To investigate the architectural parameters that dictate the substrate specificity and site-selectivity of a Rieske oxygenase catalyzed reaction, we focused on two Rieske oxygenases, SxtT and GxtA, which are involved in the biosynthesis of paralytic shellfish toxins. These enzymes share 88% sequence identity with one another and selectively install a hydroxyl group on adjacent C12 and C11 positions of a tricyclic saxitoxin scaffold, respectively. Each structure showcases an α3 trimeric architecture, and each protomer of the trimer contains a Rieske cluster in the N-terminal domain and a non-heme iron center in the C-terminal domain. The trimeric quaternary architecture places these metallocenters within electron transfer distance of one another across the subunit-subunit interfaces.

To investigate how the native hydroxylated substrates bind to SxtT and GxtA and to identify global architectural differences between these proteins, we solved the structures of SxtT and GxtA with β-STOH bound, as well as that of GxtA with STX, bound to 1.79-, 1.79-, and 1.74-Å resolution, respectively. In SxtT, the presumed native substrate β-STOH shows slight deviations in its position in the active site relative to that observed with ddSTX, but it maintains interactions with Arg204, Cys228, Gln226, Ser230, Asp239, Tyr273, and Thr276. The differentiating feature between β-STOH and ddSTX, the C12 β-hydroxyl group, forms only one additional interaction in the SxtT active site with Tyr198. This interaction is mediated by a water molecule and Tyr198, like Cys228, Asp239, and Tyr273 is conserved in GxtA. The most significant structural difference between these substrate-bound structures of SxtT and GxtA is the orientation of a loop that connects the β13 and β14 strands of the C-terminal iron-binding domain. In SxtT, this loop extends toward the active site and interacts with β-STOH as well as with non-conserved residues Ser230 and Glu272. Two of the corresponding loop residues in SxtT (Val206 and Ile209) are hydrophobic and unlikely to reside on the protein surface or form similar interactions with the corresponding surface residues Pro233 and Glu234. Accordingly, whereas both orientations of the GxtA loops reveal an open path from the surface of the protein to the substrate-binding site, the SxtT loop, which is tucked into the protein interior, blocks the analogous path in the crystal structure. Outside of considering the overall loop architecture, in SxtT, the loop is important as it interacts with a bound substrate using residue Arg204. This Arg204 interaction, coupled with additional interactions that are formed between active site residues (Thr276, Gln226, Ser230, Asp239, and Tyr273) and the guanidinium groups of the five- and six-membered rings of β-STOH, ensures that three regions of ddSTX and β-STOH are recognized by SxtT.

>[3x]MTTADLILINNWHVVANVEDCKPGSITTARLLGVKLVLWRSQEQNSPIQVWQDYCPHRGVPLSMGEVANNTLVCPYHGWRYNQAGKCVQIPAHPDMVPPASAQAKTYHCQERYGLVWVCLGNPVNDIPSFPEWDDPNYHKTYTKSYLIQASPFRVMDNSIDVSHFPFIHDGWLGDRNYTKVEDFEVKVDKDGLTMGKYQFQTSRIVSHIEDDSWVNWFRLSHPLCQYCVSESPEMRIVDLMTIAPIDEDNSVLRMLIMWNGSEMLESKMLTEYDETIEQDIRILHSQQPARLPLLAPKQINTQGLPQEIHVPSDRGTVAYRRWLKELGVTYGVC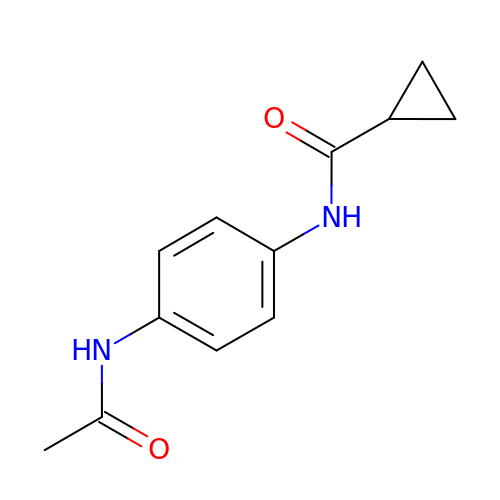N-[4-(acetylamino)phenyl]cyclopropanecarboxamide | C12 H14 N2 O2 | XJFJFROTOPBZCO-UHFFFAOYSA-N>MGHHHHHHMTQTITVIRGDGIGPEIMDATLFVLDALQAGLTYEYADAGLVALEKHGDLLPESTLASITKNKVALKSPLTTPVGEGFSSINVAMRRKFDLYANVRPAKSFPNTKSRFADGV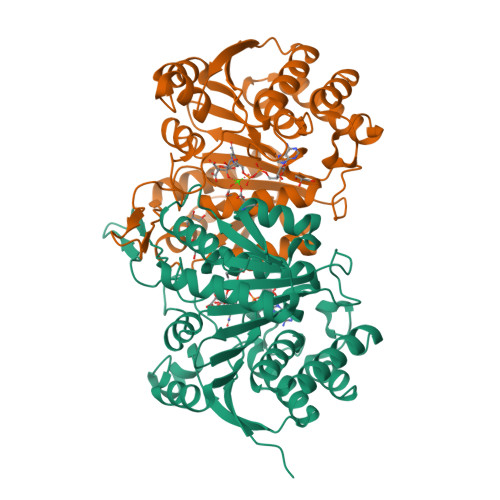DLITVRENTEGAYLSEGQEVSADGEVAVSGARVTRKGSERIVRYAFDLARATGRKKVTAVHKANIIKSTSGLFLKVARDVATQYPEIEFQEMIVDNTCMQLVMRPEQFDIIVTTNLFGDIISDLCAGLVGGLGLAPGANIGVDAAIFEAVHGSAPDIAGQGKANPCALLLGAAQMLDHIGQPQNAERLREAIVATLEAKDSLTPDLGGTGNTMGFAKAIASRL[2x]> MESTANALVVKVSYGGVLRRFRVPVKANGQLDLEMAGLKEKIAALFNLSADAELSLTYSDEDGDVVALVDDNDLFDVTNQRLKFLKINVNAGVS

PB1 domains are protein interaction modules with critical roles in the assembly of protein complexes involved in autophagy, signaling, cell division, and redox processes, as well as the auxin-response pathway in plants. PB1 domains form homotypic interactions via conserved electrostatic motifs molded by basic or acidic surface patches on opposite faces of their ubiquitin-like β-grasp fold. While type A and type B PB1 domains can form heterodimeric protein complexes, type AB members can mediate interactions with either PB1 domain type or engage in homotypic interactions to form homo-oligomers or hetero-oligomers. Our cryo-EM structures of filamentous p62 and AtNBR1–PB1 assemblies revealed that the presence of a tandem arginine sequence in the basic motif of type AB interfaces is required to stabilize a polymeric assembly.

Of the three PB1 assemblies studied, AtNBR11–94 (AtNBR1–PB1) and p621–122 (p62-PB1) formed homogeneous filaments of constant diameter that appeared best suited for high-resolution structure investigation by cryo-EM. Image classification of segmented PB1 helices revealed that both AtNBR1–PB1 and p62-PB1 polymerize in two different tubular morphologies: a projection class with a ladder-like pattern, we term L-type, and a projection class with a serpent-like one, we term S-type. By indexing the layer lines in the Fourier spectra of AtNBR1–PB1 filaments, we concluded that L-type is a two-stranded helix with a pitch of 77.2 Å and 11.47 subunits/turn, whereas S-type is a single double-stranded helix with a pitch of 68.2 Å and 11.55 subunits/turn. Using the derived symmetries, we determined the 3.5/3.9- (L-type, p62/AtNBR1) and 4.0/4.4 Å- (S-type, p62/AtNBR1) resolution structures. All four structures form tubules of ~120 Å and 150-Å width with an inner diameter of 45 Å and 70 Å for AtNBR1–PB1 and p62-PB1, respectively. In the absence of prior structural information, we traced the AtNBR1–PB1 de novo. This de novo-built model is in close agreement with the 1.6-Å crystal structure of a polymerization-deficient AtNBR1–PB1 mutant, which we solved in parallel. The main interactions are formed between a double arginine finger formed by two neighboring arginine residues in strand β2 (R19–R20AtNBR1/R21–22p62) stabilizing strong salt bridges to acidic residues (D60/D62/D64/D73AtNBR1 or D69/D71/D73/E82p62) in the OPCA motif located in the β2–β3 loop and the α2 helix. These interactions are assisted by the canonical-type B lysine (K11AtNBR1 and K7p62) in strand β1. In addition to the canonical transverse interactions, the helices are further stabilized by longitudinal interactions Y14AtNBR1/N28AtNBR1 or K102p62/D92p62 and R59p62/D93p62 to subunits of neighboring strands along the helical axis.>[2x]MSFQGHGIYYIASAYVANTRLALSEDSSANKSPDVIISSDAVDPLNNLWLIEPVGEADTYTVRNAFAGSYMDLAGHAATDGTAIIGY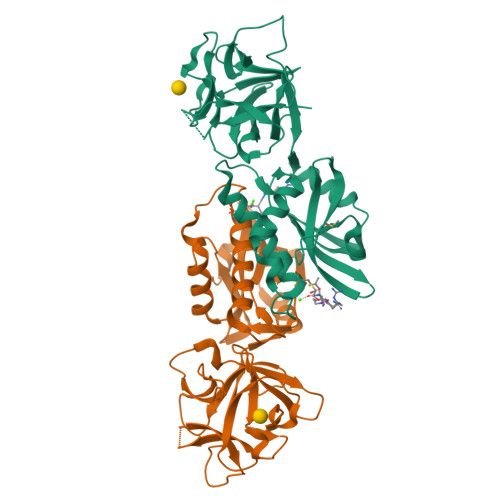RPTGGDNQKWIISQINDVWKIKSKETGTFVTLLNGDGGGTGTVVGWQNITNNTSQNWTFQKLSQTGANVHATLLACPALRQDFKSYLSDGLYLVLTRDQISSIWQASGLGSTPWRSEIFDCDDFATVFKGAVAKWGNENFKANGFALLCGLMFGSKSSGAHAYNWFVERGNFSTVTFFEPQNGTYSANAWDYKAYFGLF>KNKTIEVYVDRATLPTIQQMTQIINENSNNKKLISWSRYPINDETLLESINGSFFKNRPELIKSLDSMILTNEIKKVIINGNTLWAVDVVNIIKSIEALGKKTEIELNFYDDGSAEYVRLYDFSRLPESEQEYKISLSKDNIQSSINGTQPFDNSIENIYGFSQLYPTTYHMLRADIFETNLPLTSLKRVISNNIKQM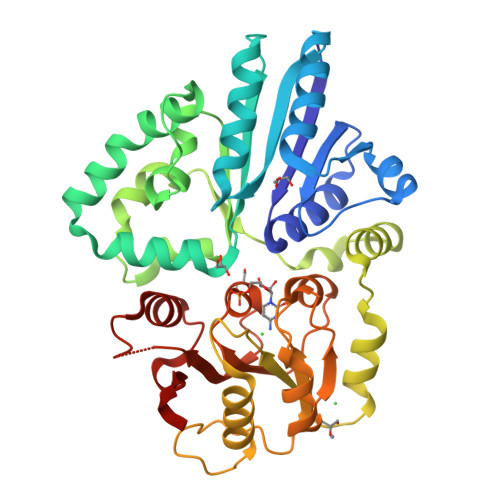KWDYFTTFNSQQKNKFYNFTGFNPEKIKEQYKASPHENFIFIGTNSGTATAEQQIDILTEAKKPDSPIITNSIQGLDLFFKGHPSATYNQQIIDAHNMIEIYNKIPFEALIMTDALPDAVGGMGSSVFFSLPNTVENKFIFYKSDTDIENNALIQVMIELNIVNRNDVKLISDLQ[2x]> GPTVGGQLGTAGQGFSYSKSNGRGGSQAGGSGSAGQYGSDQQHHLGSGSGAGGTGGPAGQAGRG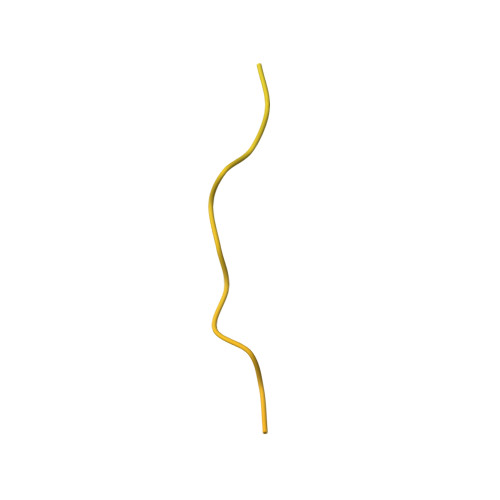GAAGTAGVGETGSGDQAGGEGKHITVFKTYISPWERAMGVDPQQKMELGIDLLAYGAKAELPKYKSFNRTAMPYGGYEKASKRMTFQMPKFDLGPLLSEPLVLYNQNLSNRPSFNRTPIPWLSSGEPVDYNVDIGIPLDGETEEL>[4x]MTKIFAYAIREDEKPFLKEWEDAHKDVEVEYTDKLLTPETVALAKGADGVVVYQQLDYIAETLQALADNGITKMSLRNVGVDNIDMAKAKELGFQITNVPVYSPNAIAEHAAIQAARILRQDKAMDEKVARHDLRWAPTIGRE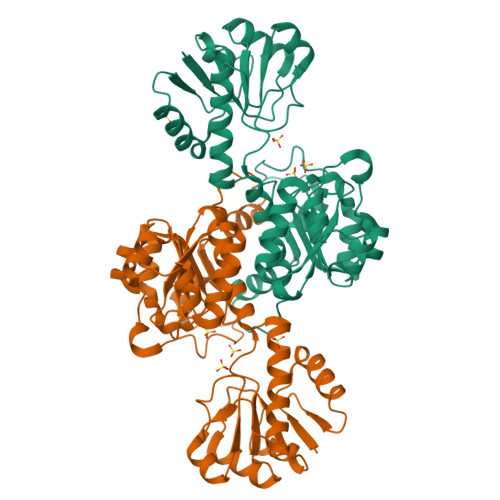VRDQVVGVVGTGHIGQVFMQIMEGFGAKVITYDIFRNPELEKKGYYVDSLDDLYKQADVISLHVPDVPANVHMINDESIAKMKQDVVIVNVSRGPLVDTDAVIRGLDSGKIFGYAMDVYEGEVGIFNEDWEGKEFPDARLADLIARPNVLVTPKTAFYTTHAVRNMVVKAFDNNLELVEGKEAETPVKVG> GSVLVIRI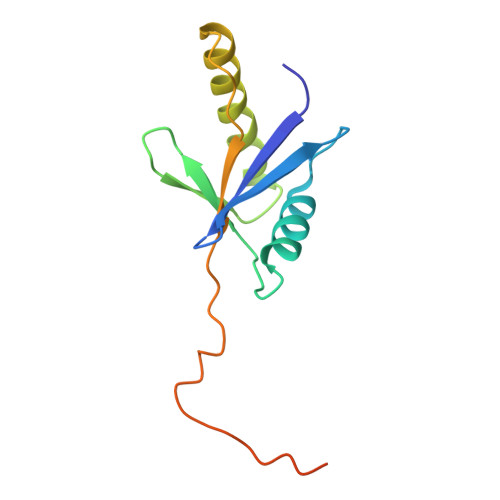KIPNSGAVDWTVHSGPQLLFRDVLDVIGQVLPEATTTAFEYEDEDGDRITVRSDEEMKAMLSYYYSTVMEQQVNGQLIEPLQIFPRACKPPGERNIHGLKVNTRAGPSQSGRHHHHHH>[2x]FQGPLGSHMTISPKEKEKIAIHEAGHALMGLVSDDDDKVHKISIIPRGMALGVTQQLPIEDK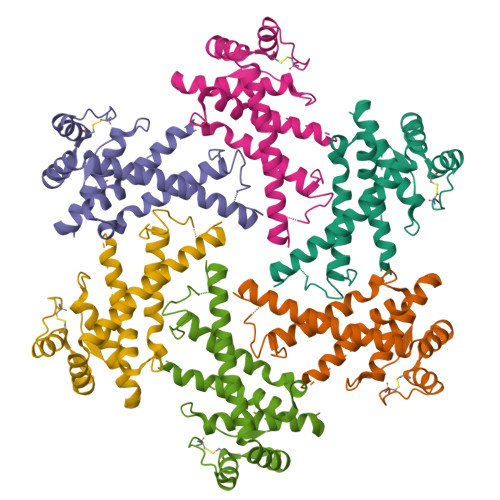HIYDKKDLYNKILVLLGGRAAEEVFFGKDGITTGAENDLQRATDLAYRMVSMWGMSDKVGPIAIRRVANPFLGGMTTAVDTSPDLLREIDEEVKRIITEQYEKAKAIVEEYKEPLKAVVKKLLEKETITCEEFVEVFKLYGIELKDKCKKEELFDKDRKSEENKELKSEEVKEEVV>[2x]MIDQSDWISFSHMSSDTDHFPIKSWFRCEQKAASRSYRTLGDMSHPQGIYEVRAAITRLISLTRGVKCRPEQMIIGAGTQVLMQLLTELLPKEAVYAMEEPGYRRMYQLLKNAGKQVKTIMLDEKGMSIAEITRQQPDVLVTTPSHQFPSGTIMPVSRRIQLLNWAAEEPRRYIIEDDYDSEFTYDVDSIPALQSLDRFQNVIYMGTFSKSLLPGLRI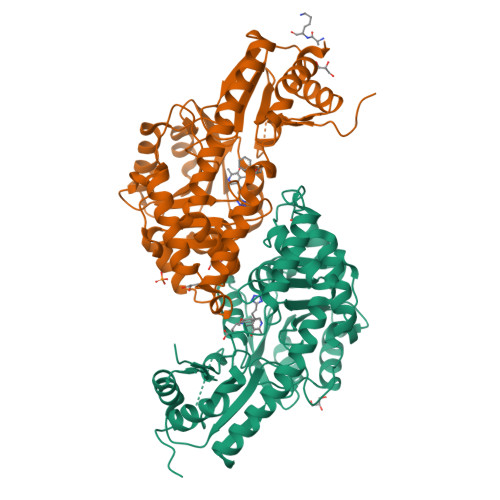SYMVLPPELLRAYKQRGYDLQTCSSLTQLTLQEFIESGEYQKHIKKMKQHYKEKRERLITALEAEFSGEVTVKGANAGLHFVTEFDTRRTEQDILSHAAGLQLEIFGMSRFNLKENKRQTGRPALIIGFARLKEEDIQEGVQRLFKAVYGHKKIPVTGDHHHHHH> NGDRLYRADSRPPDEIKRSGGLMP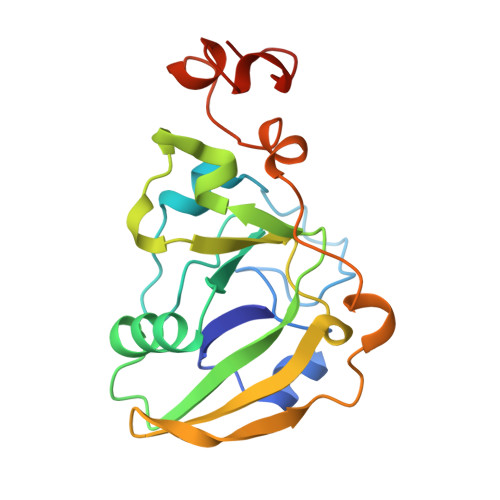RGHNEYFDRGTQMNINLYDHARGTQTGFVRYDDGYVSTSLSLRSAHLAGQSILSGYSTYYIYVIATAPNMFNKNDVLGVYSPHPYEQEVSALGGIPYSQIYGWYRVNFGVIDERLHRNREYRDRYYRNLNIAPAEDGYRLAGFPPDHQAWREEPWIHHAPQGCGNSS> GPGDQRFGDLVFRQLAPNVWQHTSYLDMPGFGAVAS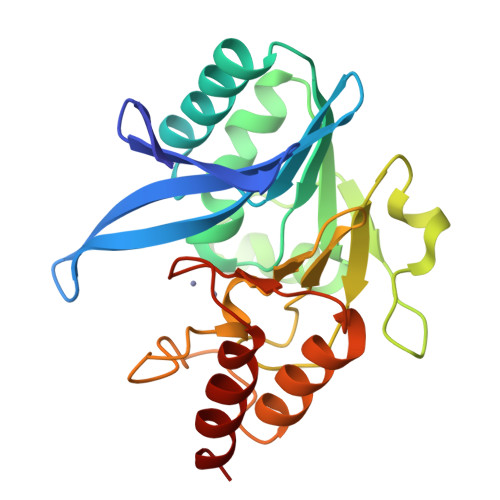NGLIVRDGGRVLVVDTAWTDDQTAQILNWIKQEINLPVALAVVTHAHQDKMGGMGALHAAGIATYANALSNQLAPQEGLVAAQHSLTFAANGWVEPATAPNFGPLKVFYPGPGHTSDNITVGIDGTDIAFGGCLIKDSKAKSLGNLGDADTEHYAASARAFGAAFPKASMIVMSHSAPDSRAAITHTARMADKLR> MDYVIIQSMDKEVEEILTDIDYGSFSYDYEKNT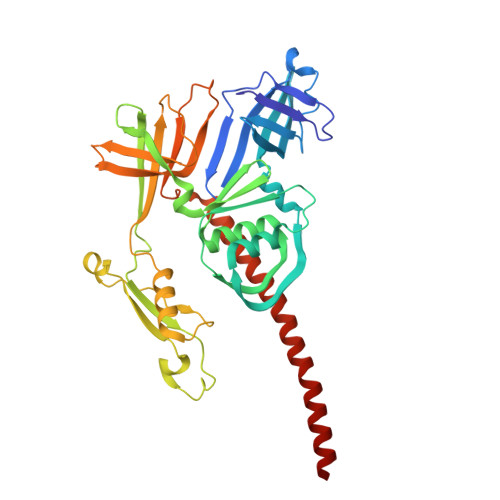SRAISFTVNKTKQNAAIFDLVGNEAILTYQGQQFVIKKCTPKSIGGTISKQITAQHICYTVQDHVQYNVKSGRKKYSIQTVLEFALQDNVLGFSYEIQGSFPLVELEDLGNKNGLELVNLCLEEFGAILFADNKKLYFYDEKSWYVRTEKQFRYLYNTEEVSVDTNTDNLKTEIKCYGKQKENADKLTGDNKYMAVVTYTSPNEAIYGKRMANAKSDDKITNNDDLLIFAKKQILDVPETALTIAYKGKEPVSERDVWYFIHEPMGFETEVKVTKIKSSHPWSKKFQEIGFSNSRRDMVRIQTQIANQVKKASVDTNKINSFSSIAMNAYDSRILTEVVGVVDGD>SNARDPRPLRDKNFQSAIQEEIYDYLKKNKFDIETNHPISIKFLKQPTQKGFIIIFKWLYLRLDPGYGFTKSIENEIYQILKNLRYPFLESINKSQISAVGGSNWHKFLGMLHWMVRTNIKLDMCLNKVDRSLINQNTQEITILSQPLKTLDEQDQRQERYELMVEKLLIDYFTESYKSFLKLEDNYEPSMQELKLGFEKFVHIINTDVTSTELKLEELKVDLNRKRYKLHQQVIHVIDITSKFKINIQSSLENSENELGNVIEELRNLEFE[2x];>MTSRINKPWRISHSPNSKIPSPVREKLNRLSRNQDVFPILDLQELVICLQSCDFALATQENISRPTSDYMVTLYKQIIENFMGISVESLLNSSNQETGDGHLQEENENIYLDTLNVLVLNKICFKFFENIGVQDFNMTDLYKPEAQRTQRLLSAVVNYARFREERMFDCNSFILQMESLLGQINKLNDEIKQLQKDFEVEVKEIEAAYSLLSGHINKYMNEMLEYMQ[2x];>MSQKDNLLDNPVEFLKEVRESFDIQQDVDAMKRIRHDLDVIKEESEARLKLYRSLGVILDLENDQVLINRKNDGNIDILPLDNNLSDFYKTKYIWERLG[2x];>MASIDAFSDLERRMDGFQKDVAQVLARQQNHVALYERLLQLRVLPGASDVHDVRFVFGDDSRCWIEVAMHGDHVIGNSHPALDPKSRATLEHVLTVQGDLAAFLVVARDMLLAS[2x]

Ndc80c, a heterotetramer of Ndc80, Nuf2, Spc24, and Spc25, is a 600 Å long rod, largely two-chain coiled-coil, with an Ndc80/Nuf2 globular “head” at one end and an Spc24/Spc25 globular knob at the other. The Mps1 and Aurora B kinases regulate and monitor kinetochore attachment to spindle microtubules during cell division, ultimately ensuring accurate chromosome segregation. We show here, biochemically and structurally, that short peptide segments on both Mps1 and Ipl1 bind the site on the Ndc80/Nuf2 head of Ndc80c that we have shown previously to bind an Ipl1-phosphoregulated peptide segment near the C-terminus of Dam147. The Ndc80c head is thus a communication hub for ensuring a robust linkage between centromere and spindle and for integrating the SAC with tension sensing and error correction.

We generated a chimeric construct that fused to the N-terminus of Ndc80cdwarf Nuf2 a peptide containing Ipl1 residues 26–59, with 40–44 (a disordered loop in the AF2 prediction) deleted. The chimera crystallized in space group P43212 (a = b = 115Å, c = 424Å), with two complexes in the asymmetric unit related by an approximate non-crystallographic dyad. We recorded anisotropic diffraction data to a minimum Bragg spacing of 3.9Å, but intensities of reflections in the a* and b* directions fell below significance at Bragg spacings of ~6 Å. When phased only on the molecular-replacement model, a difference map showed strong density for ordered parts of the Ipl1 segment and a structure overall that was consistent with the AF2 prediction between Ipl1 residues 48 and 56. The density for this segment was continuous with that for the Nuf2 subunit of the non-crystallographic-symmetry related complex. Thus, the asymmetric unit is a “domain-swapped” dimer, and the interactions may have been essential for the crystals to form, suggesting that the interaction might occur in solution. Although both sequence alignment and AF2 prediction suggest a potential first part of a bipartite motif, the density map was not continuous enough in the predicted region to build any structure with confidence. The refined conformation of the peptide between residues 50 and 56 (or 76 and 82) is very similar to that of the Mps1 motif, and hence also to the Dam1 peptide, even though the starting point for fitting the peptide was independent of the Mps1 and Dam1 structures. The second-part binding motif, SKIPSP(V/I)R, is present with some variation, in Ipl1/AuroraB from other point-centromere yeast. The Ipl1 peptide bound more weakly than those from Dam1 and Mps1, but avidity contributed by the two copies of the conserved motif might enhance binding of the intact protein.PUF proteins, named for PUM (Pumilio) and FBF (fem-3 binding factor), are an exemplary system for understanding the divergence of RNA recognition within eukaryotic RNA-binding protein families. Eight PUM repeats are arranged in a crescent shape with the RNA bound on the concave face of the protein. Each repeat contributes a trio of amino acid residues, termed a tripartite recognition motif (TRM), that directly contact the opposing RNA base. FBF recognizes a 9-nt motif, 5´-UGURNNAUA-3´, whereas PUF-8 binds an 8-nt sequence, 5´-UGUANAUA-3´.

First, we addressed whether the serine residues that occupy edge-on positions are required to confer preference of the PBE. We substituted alanine for one (AS/Y or SA/Y) or both (AA/Y) of the edge-on serine residues. Intriguingly, all of the mutants with edge-on alanine substitutions and a tyrosine stacking residue retained preferential binding to the 8-nt PBE over the 9-nt FBE. A crystal structure of the AS/Y variant in complex with PBE RNA was nearly identical to the SS/Y structure. FBF-2 R5 SS/Y bound equally well to either an A or G at position 4, similar to WT FBF-2, and the R5 AS/Y variant accommodated A4, G4 or U4. The tyrosine base-stacking interaction is critical for binding energy, whereas serine or alanine residues in the edge-interacting positions permit binding to different nucleotides at position 4.

> GSNNVLPTWSLDSNGEMRSRLSLSEVLDSGDLMKFAVDKTGCQFLEKAVKGSLTSYQKFQLFEQVIGRKDDFLKLSTNIFGNYLVQSVIGISLATNDDGYTKRQEKLKNFISSQMTDMCLDKFACRVIQSSLQNMDLSLACKLVQALPRDARLIAICVDQNANHVIQKVVAVIPLKNWEFIVDFVATPEHLRQICSDKYGAYVVSTIIEKLTADSMNVDLTSAAQNLRERALQRLMTSVTNRCQELATNEYANYIIQHIVSNDDLAVYRECIIEKCLMRNLLSLSQEKFASHVVEKAFLHAPLELLAEMMDEIFDGYIPHPDTGKDALDIMMFHQFGNYVVQCMLTICCDAVSGRRQTKEGGYDHAISFQDWLKKLHSRVTKERHRLSRFSSGKKMIETLANLRSTHPIYELQ>GHMNTRNFSLPQLQNLPIEEARIVADALAVHATSRQIDSAASKLAALAEAGLKGDRQAYAAYQQLLYVLSLSDDVATAQTRRWLARAIYRVEERFMPAADLSRALSEEDFQKRLEQEIAAQSRERHPMSQYVFSGSASRAQLQVFLRHQWFRTFRLYRDAADLLVNLTDVDEAAALARYLYGELGEEDEKGSHPRLLAKLLEAIGLEADFQAVSTMPEEIAYLNNRARAFRHAEVGWGLAVFY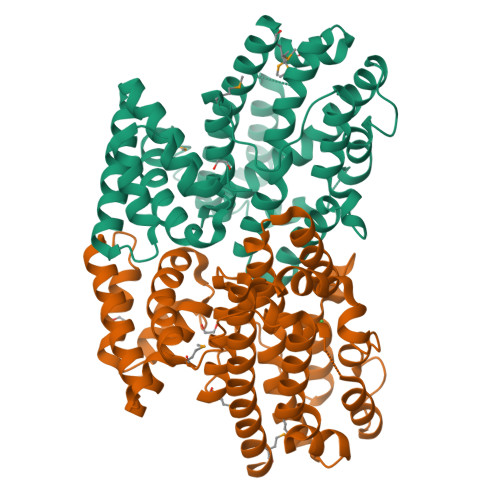ITELVVPGNHEKLYRALLQAGLSEDQAEYYKVHISLVPPRAKREWQLIARRIPDVQFQNAFLTSLSQHFRVERAYYDAIWEEMQSVKGS[3x]ASPARAGINE 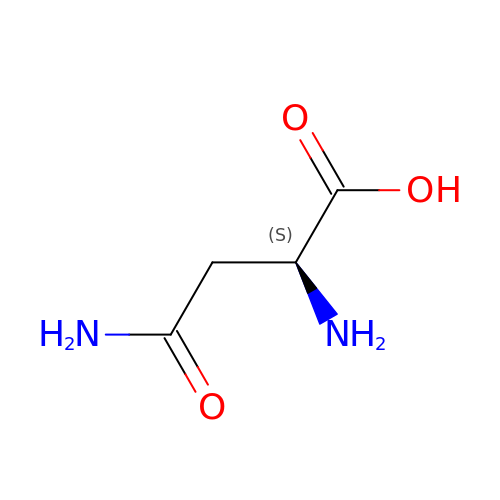| C4 H8 N2 O3 | DCXYFEDJOCDNAF-REOHCLBHSA-N>MAAALSEQLAELEKRSGGRLGVAVLDTATGRRFGYRGDERFPMCSTFKALLAAAVLARVDQGKENLDRRITYGKEDLVDYSPVTEKHVGDGMTVAELCEAAITYSDNTAANLLLEALGGPAALTAFLRSIGDNVTRLDRWEPELNTAAPGDPRDTTTPAAMAATLRTLLLGDVLSPASRQQLVDWLIANKTGDKRLRAGLPADDRVGDKTGTGEHGTTNDIAVVWPPNRAPIFLAVYLTESQVDADARDAVIAEVARLVVAAWLHHHHH[3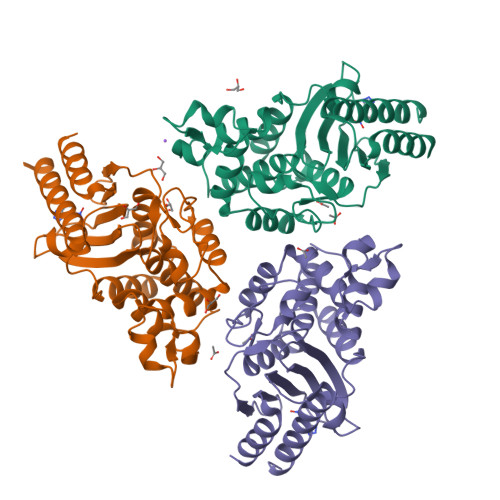x]>[2x]TRKTYTLTDYLKNTYRLKLYSLRWISDHEYLYKQENNILVFNAEYGNSSVFLENSTFDEFGHSINDYSISPDGQFILLEYNYVKQWRHSYTASYDIYDLNKRQLITEERIPNNTQWVTWSPVGHKLAYV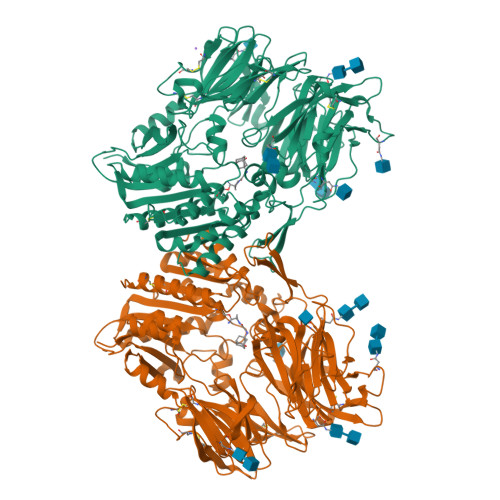WNNDIYVKIEPNLPSYRITWTGKEDIIYNGITDWVYEEEVFSAYSALWWSPNGTFLAYAQFNDTEVPLIEYSFYSDESLQYPKTVRVPYPKAGAVNPTVKFFVVNTDSLSSVTNATSIQITAPASMLIGDHYLCDVTWATQERISLQWLRRIQNYSVMDICDYDESSGRWNCLVARQHIEMSTTGWVGRFRPSEPHFTLDGNSFYKIISNEEGYRHICYFQIDKKDCTFITKGTWEVIGIEALTSDYLYYISNEYKGMPGGRNLYKIQLSDYTKVTCLSCELNPERCQYYSVSFSKEAKYYQLRCSGPGLPLYTLHSSVNDKGLRVLEDNSALDKMLQNVQMPSKKLDFIILNETKFWYQMILPPHFDKSKKYPLLLDVYAGPCSQKADTVFRLNWATYLASTENIIVASFDGRGSGYQGDKIMHAINRRLGTFEVEDQIEAARQFSKMGFVDNKRIAIWGWSYGGYVTSMVLGSGSGVFKCGIAVAPVSRWEYYDSVYTERYMGLPTPEDNLDHYRNSTVMSRAENFKQVEYLLIHGTADDNVHFQQSAQISKALVDVGVDFQAMWYTDEDHGIASSTAHQHIYTHMSHFIKQCFSLP> KMAKDSKAPVVEIFDERDGCTSAGSTGKASDAGEKG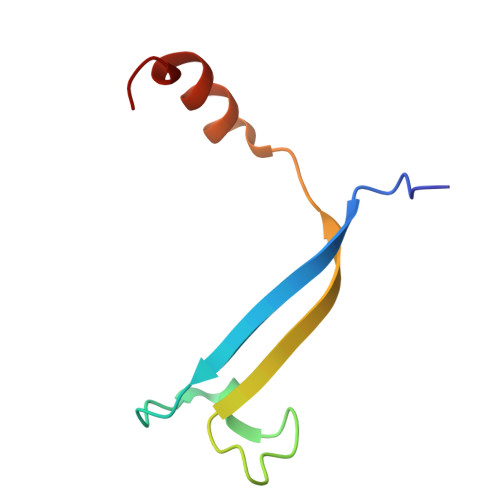LLVKVSMQKVGYNAIMAKSVAASYMNK>MDLTVEPNLHSLITSTTHKWIFVGGKGGVGKTTSSCSIAIQMALSQPNKQFLLISTDPAHNLSDAFGEKFGKDARKVTGMNNLSCMEIDPSAALKDMNDMAVSRANNNGSDGQGDDLGSLLQGGALADLTGSIPGIDEALSFMEVMKHIKRQEQGEGETFDTVIFDTAPTGHTLRFLQLPNTLSKLLEKFGEITNKLGPMLNSFMGAGNVDISGKLNELKANVETIRQQFTDPDLTTFVCVCISEFLSLYETERLIQELISYDMDVNSIIVNQLLFAENDQEHNCKRCQARWKMQKKYLDQIDELYEDFHVVKMPLCAGEIRGLNNLTKFSQFLNKEYNPI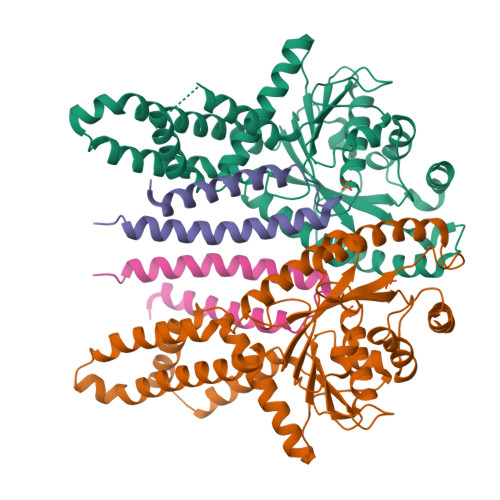TDGKVIYELEDKELEHHHHHH[5x];>MNELSKKYLAKVKERHELKEFNNSISAQDNYAKWTKNNRKLDSLDKEINNLKDEIQSENHHHHHH[5x]>[2x]GVSGSKGQKLFVSVLQRLLSERGLHVKESSAIE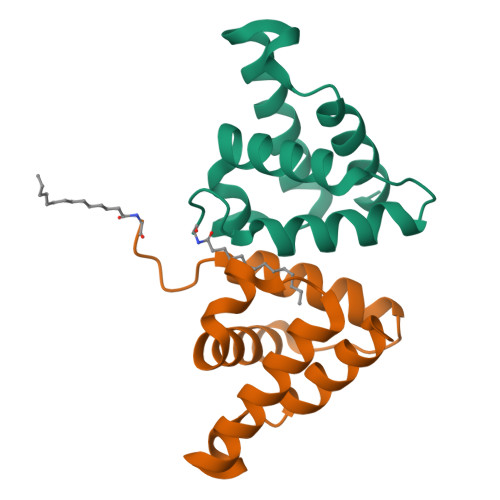FYQFLIKVSPWFPEEGGLNLQDWKRVGREMKRYAAEHGTDSIPKQAYPIWLQLREILT> ATSSPSTTPINFHINKPFVFA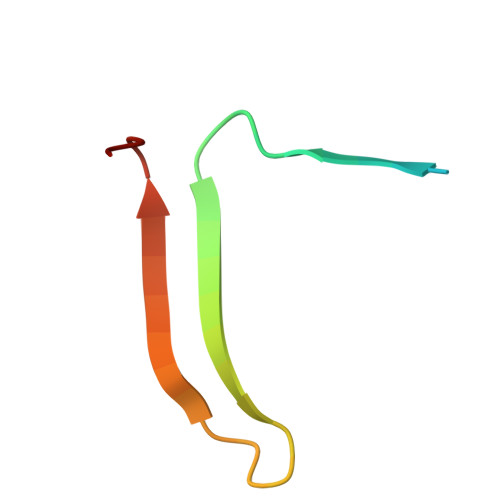IREKSTGVILFIGEIGEVKE> MAESPIGVVVSSRRNGPWAELTLVLTPQELDQGKRLLLGELVRVSSGGKDYVGMVLDGYYEPVGRSDPTYTLALAHINQVDLEKEDPWARKEVNFYHHRIVLLGRVVQGGLFAPSTRLLPPVVEARVYRMTEEELQRLLAAEVRTSGSVKAEGKRRYAFGHLAYGLEEGGEYPEVVKEVDPALFVGRRTANFGKT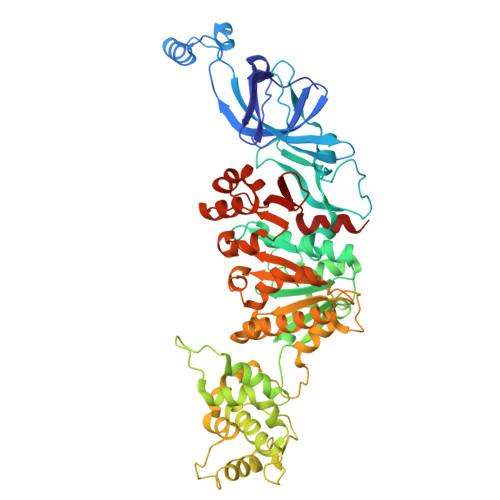GFGKSNENKVILTLLAHAFPRVGMLILDQNAEYLLQTEATTSPGLAQAFKALGIRGRIRFYTAREEAWARRLKEHLGTEWREYVEVLPLKVDFYHFPELAVALAYQRRRLQGAEPPQYLENAFYNLEDWKHIPDRMAYVYGALRKAGLTPRKGLKIKYKNENYDISEEKSWGNLQEAMENNSQRGDNKGGARELYSRAKVFSFLRAFHAPGKEANFLETIKEDLLGEKTEGEGKVVILDLPSLGEAADFFTLRLMDLLFDRAVELYGKRQANFLVVLEEAHNFLEDKAGIFYRVAKEGRKYGIGMLYSTQSPASIPMEILSQTENFLVKHLSSEEDVKVLKRAKAPFAFVADFLLSEPIIGYSYVYFEPYQPFVVPLRVKLLEHVLKSLDS>[12x]MNYATVNDLCARYTRTRLDILTRPKTADGQPDDAVAEQALADASAFIDGYLAARFVLPLTVVPSLLKRQCCVVAWFYLNESQPTEQITATYRDTVRWLEQVRDGKTDPGVESRTAASPEGEDLVQVQSDPPVFSRKQKGFI;>MGRILDISGQPFDFDDEMQSRSDELAMVMKRTQEHPSSGVTPNRAAQMLRDAERGDLTAQADLAFDMEEKDTHLFSELSKRRLAIQALEWRIAPARDASAQEKKDADMLNEYLHDAAWFEDALFDAGDAILKGYSMQEIEWGWLGKMRVPVALHHRDPALFCANPDNLNELRLRDASYHGLELQPFGWFMHRAKSRTGYVGTNGLVRTLIWPFIFKNYSVRDFAEFLEIYGLPMRVGKYPTGSTNREKATLMQAVMDIGRRAGGIIPMGMTLDFQSAADGQSDPFMAMIGWAEKAISKAILGGTLTTEAGDKGARSLGEVHDEVRREIRNADVGQLARSINRDLIYPLLALNSDSTIDINRLPGIVFDTSEAGDITALSDAIPKLAAGMRIPVSWIQEKLHIPQPVGDEAVFTIQPVVPDNGSQKEAALSAEDIPQEDDIDRMGVSPEDWQRSVDPLLKPVIFSVLKDGPEAAMNKAASLYPQMDDAELIDMLTRAIFVADIWGRLDAAADH[12x]

Myophage Mu is a representative of contractile nanomachines with a simple tail baseplate. It has the capacity to infect a range of intestinal bacteria and has extensive applications in genetic engineering research. Using cryo-EM, we resolved the three-dimensional (3D) structures of the G(+) type phage Mu in both its extended state and urea-induced contracted state, the latter lacking the baseplate, at near-atomic resolutions. The structure of extended Mu can be divided into four distinct regions: the DNA-containing head, the connector complex, the tail, and the baseplate.

By employing the symmetry mismatch reconstruction and the local reconstruction methods, the structures of the portal-adaptor and the terminator-tail region of extended Mu were resolved to resolutions of 3.4 Å and 3.5 Å, respectively. The Mu connector complex, which attaches the tail to the icosahedral head, is comprised of three proteins: the portal protein gp29, the adaptor protein gp36, and the tail terminator protein gp37. The connector complex in the majority of myophages and siphophages contains the portal, adaptor (the first head-tail joining protein), stopper (the second head-tail joining protein), and tail terminator protein, but Mu is the rarely reported myophage to possess only the first head-tail joining protein. The Mu portal is constituted of 12 copies of the protein gp29. Each gp29 protein contains four distinct domains: a crown domain, a wing domain, a stem domain, and a clip domain. It is noteworthy that the final 124 residues of the C-terminus in gp29 are absent in our structure, which verifies that its C-terminus may undergo proteolytic cleavage by protease I during head assembly. The Mu adaptor is constituted by 12 copies of the protein gp36, each of which comprises an α-helix domain and an elongated C-arm. The C-arm of Mu gp36, which is absent in the X-ray structure, is inserted into the clip domain of the portal to form an extended four-stranded β-sheet, thereby further stabilizing the interactional interface between the portal and adaptor. The adaptor gp36 exhibits structural similarities to that observed in siphophages and myophages, with their α-helix domains adopting substantial structural similarity, but their C-arms and β-hairpins exhibiting conformational differences, possibly due to the differences in their structural environment. Despite lacking the stopper, the adaptor of Mu, which may assume the stopper function, serves as a docking platform by binding to the tail terminator protein to join the head and tail and prevents the release of the genome.N~2~-(AMINOCARBONYL)-N~1~-{4-{[AMINO(IMINO)METHYL]AMINO}-1-[HYDROXY(1,3-THIAZOL-2-YL)METHYL]BUTYL}VALINAMIDE 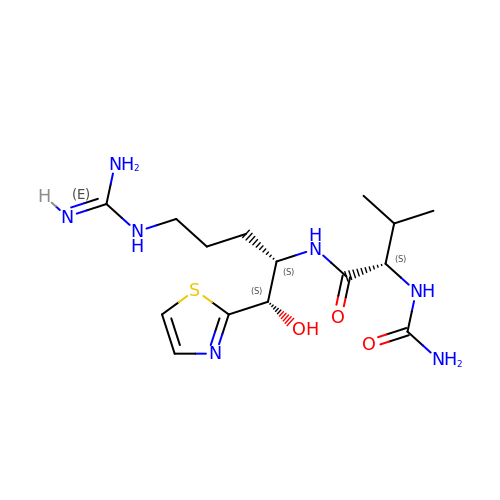| C15 H27 N7 O3 S | WOLWXHDYZAKRKB-DCAQKATOSA-N> APLAQANSIKVSVSSGGDCVRTYRPEIKKGSYNNIVVHVKTAVADNLLFYLGSAKFIDFLAIEMRKGKVSFLWDVGSGVGRVEYPDLTIDDSYWYRIEASRTGRNGSISVRALDGPKASMVPSTYHSVSPPGYTILDVDANAMLFVGGLTGKIKKADAVRVITFTGCMGETYFDNKPIGLWNFREKEGDCKGCTVSPQVEDSEGTIQFDGEGYALVSRPIRWYPNISTVMFKFRTFSSSALLMYLATRDLKDFMSVELSDGHVKVSYDLGSGMTSVVSNQNHNDGKWKAFTLSRIQKQANISIVDIDSNQEENVATSSSGNNFGLDLKADDKIYFGGLPTLRNLRPEVNVKKYSGCLKDIEISRTPYNILSSPDYVGVTKGCSLENVYTVSFPKPGFVELAAVSIDVGTEINLSFSTRNESGIILLGSGGGQAYYAIFLNKGRLEVHLSSGTRTMRKIVIKPEPNRFHDGREHSVHVERTRGIFTVQIDEDRRHMQNLTEEQPIEVKKLFVGGAPPEFQPSPLRNIPAFQGCVWNLVINSIPMDFAQPIAFKNADIGRCTYQKPREDESEAVPAEVIVQP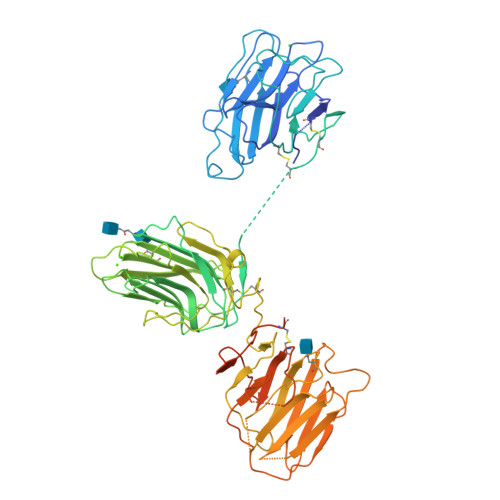QPVPTPAFPFPAPTMVHGPAAAHHHHHH> LKPYCRPSTSVVLQGLPMVARKTLFMLPDGGGSAFSYASLPRLKSDTAVVGLNCPYARDPE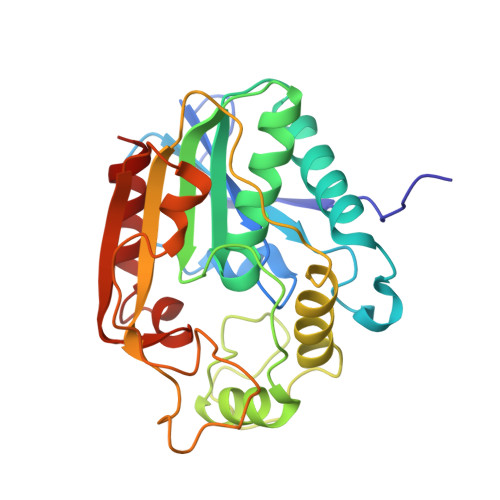NMNCTHGAMIESFCNEIRRRQPRGPYHLGGWSSGGAFAYVVAEALVNQGEEVHSLIIIDAPIPQAMEQLPRAFYEHCNSIGLFATQPGASPDGSTEPPSYLIPHFTAVVDVMLDYKLAPLHARRMPKVGIVWAADTVMDERDAPKMKGMHFMIQKRTEFGPDGWDTIMPGASFDIVRADGANHFTLMQKEHVSIISDLIDRVMA> MRDRQAFERAKDLQAVIFDKTGTLTEGRFGVTDIVGFNHSEDELLQIAASLEARSEHPIAAAIVEEAEKRGFGLTEVEEFRAIPGKGVEGIVNGRRYMVVSPGYIRELGIKTDESVEKLKQQGKTVVFILKNGEVSGVIALADRIRPESREAISKLKAIGIKCMMLTGDNRFVAKWVAEELGLDDYFAEVLPHEKAEKVKEVQQKYVTAMVGDGVNDAPALAQADVGIAIGAGTDVAVETADIVLVRNDPRDV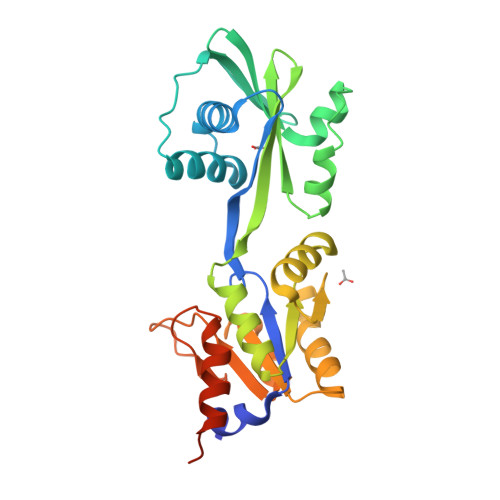AAIVELSRKTYSKFHGLSAWSHPQFEK>DWPVYHRIDGPIVMIGFGSIGRGTLPLIERHFAFDRSKLVVIDPSDEARKLAEARGVRFIQQAVTRDNYRELLVPLLTAGPGQGFCVNLSVDTSSLDIMELARENGALYIDTVVEPWLGFYFDPDLKPEARSNYALRETVLAARRNKPGGTTAVSCCGANPGMVSWFVKQALVNLAADLGVTGEEPTTREEWARLAMDLGVKGIHIAERDTQRASFPKPFDVFVNTWSVEGFVSEGLQPAELGWGTFERWMPDNARGHDSGCGAGIYLLQPGANTRVRSWTPTAMAQYGFLVTSNESISIADFLTVRD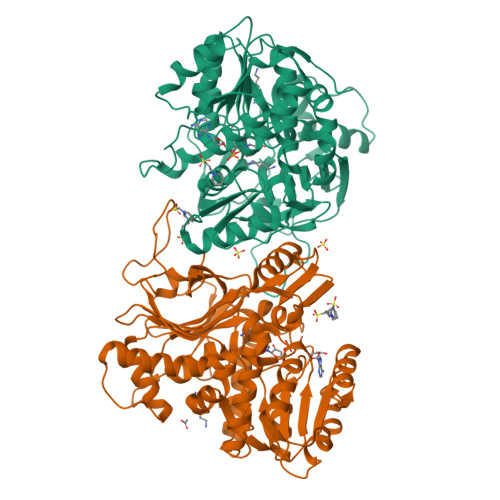AAGQAVYRPTCHYAYHPCNDAVLSLHEMFGSGKRQSDWRILDETEIVDGIDELGVLLYGHGKNAYWYGSQLSIEETRRIAPDQNATGLQVSSAVLAGMVWALENPNAGIVEADDLDFRRCLEVQTPYLGPVVGVYTDWTPLAGRPGLFPEDIDTSDPWQFRNVLVR[2x]Cobalamin-dependent methionine synthase (MS) is a key enzyme in methionine and folate one-carbon metabolism. MS is a large multi-domain protein capable of binding and activating three substrates: homocysteine, folate, and S-adenosylmethionine for methylation. Achieving three chemically distinct methylations necessitates significant domain rearrangements to facilitate substrate access to the cobalamin cofactor at the right time. Here, we use a thermophilic MS homolog (tMS) as a functional MS model.

To that end, we crystallized full-length 132 kDa tMS in its apo-form and solved the structure to 2.78 Å resolution. tMS adopts a compact, wreath-like form, and each domain aligns well with previously determined structures of equivalent excised domain or tridomain constructs. The original apo-full-length structure reveals the global orientation of each domain, resembling the reactivation conformation (Act-On) and displaying the flexibility associated with the linker regions that connect each module. The active site of the helmet-shaped Act domain is positioned above the Cob domain, where the cofactor would sit, similar to the position of these domains as previously determined with the structure of the C-terminal MS fragment, that includes the Cap, Cob, and Act domains, trapped in the reactivation conformation. Notably, tMS crystallized in the apo-form; despite the absence of Cbl, the Cob domain retains the same Rossmann-fold demonstrated by the superposition of apo-tMS Cob domain with the Cbl-bound Cob domain of E. coli MS structures that have so far been determined. The four helical bundle Cap domain is displaced ~25 Å from the resting Cap-on state and virtually identical in form and position to previously captured Cap-off structures. As such, cofactor entry is not occluded and its binding site is solvent accessible, with the Cob domain found to be preformed and ready to bind Cbl requiring minimal rearrangements. The tandem TIM-barrel Hcy and Fol domains are poised adjacently, separate from the Cob:Act domains and align well with previous structures of either the excised Fol domain or with the N-terminal fragment consisting of the Hcy and Fol domains. The edge of the Hcy domain rests against the distal side of the Act domain, forming extensive interdomain contacts through >25 hydrogen bonds and salt bridges resulting in a buried surface area of ~900 Å. Two out of four linker regions, Lys649-Asp657 (Linker II, Fol:Cap) and Glu877-Ala897 (Linker IV, Cob:Act) could not be modeled due to a lack of sufficient electron density, though the other linker regions, Pro342-Asn352 (Linker I, Hcy:Fol) and Met741-Gly747 (Linker III, Cap:Cob), could be modeled. As the only structure obtained for any B12-dependent methionine synthase in its apo-form, this structure gives a unique insight into the potential domain movements required prior to and once cobalamin is loaded.

> AKKFPYLKALLERPLVFDGAMGTELQKRDLTPEDYGGEAYFGCPEVLNRTRPEVVREIHLAYLEAGAEVIETNTFGALRHVLAEYGLEEAAEELAFLGARIAREAADPHGAFVAGALGPGTKLVSLGQISWDALYRAYKEAARGLLKGGVDLILLETAQDILQVRCAVLAVREAMAEVGREVPLQVQVTFEATGTMLVGTDEQAALAALESLPVDVVGMNCATGPDLMDSKVRYFAEHSTRFVSCLPNAGLPRNEGGRVVYDLTPEELAKWHLKFVAEYGVNAVGGCCGTGPEHIRKVAEAVKGLAPKPRPESFPPQVASLYQAVSLKQEASLFLVGERLNATGSKRFREMLFARDLEGILALAREQVEEGAHALDLSVAWTGRDELEDLRWLLPHLATALTVPVMVDSTSPEAMELALKYLPGRVLLNSANLEDGLERFDRVASLAKAHGAALVVLAIDEKGMAKTREEKVRVALRMYERLTEHHGLRPEDLLFDLLTFPITQGDEESRPLAKETLLAMEELRERLPGVGFVLGVSNVSFGLKPRARRVLNSVFLDEARKRGLTAAIVDAGKILPISQIPEEAYALALDLIYDRRKEGFDPLLAFMAYFEAHKEDPGKREDAFLALPLLERLKRRVVEGRKQGLEADLEEALKAGHKPLDLINGPLLAGMKEVGDLFGAGKMQLPFVLQAAEVMKRAVAYLEPHMEKKGEGKGTLVLATVKGDVHDIGKNLVDIILSNNGYRVVNLGIKVPIEEILKAVEAHKPHAVGMSGLLVKSTLVMKENLEYMRDRGYTLPVILGGAALTRSYVEELRAIYPNVYYAEDAFEGLRLMEELTGHAPPELTRKAPARPKREAPKVAPRARPVGEAPAVPRPPFFGVRVEEGLDLATIAHYVNKLALYRGQWGYSRKGLSREAWQALVEREAEPVFQRLLKEAMAEGWLEPKVLYGFFPVAREGEELLVFSPETGEVLERFRFPRQKGGGLSLVDYFRPRFAAPLGDEADWMPKEAFRAGARDVLGVQLVTMGEAPSRKAQALFASGAYQDYLFVHGFSVEMTEALAEYWHKRMRQMWGIAHQDATEIQKLFQQGYQGARYSFGYPACPDLADQAKLDRLMGFHRVGVRLTENFQLEPEHATSALVVHHPEARYFSVD> MGLPKGLQFFLLALLAMPMVGTQAQTAVTAEHWVDSCADWDAWDKPGPPFRVLGNTYYVGTCGIAAILITGDAGHVLIDSGTDRGAVIVRDNIARLGFSLSDVKILLHSHEHIDHVGGMASLQSLSGATLYASPAAAAVMRNGTAGEDDPQAGALASFPVARVGGLVNDGDQIALGNLRLTAYATPGHTPGALSWQWRACEEDRCTTLVYADSLSPVSAEGYRFNAHPEYLQAYRLGLATLADLECDLLLTPHPSASQMRQRLSER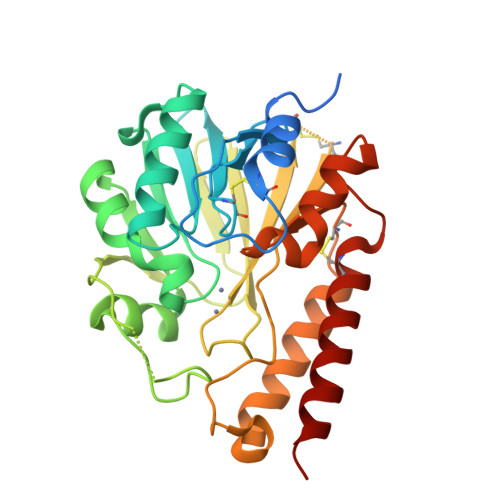QSLAVPDACRQYATGISARLAQRLASEAD> MTERTLKVLSPLHIGTGNELTPVDIYPRENIIHVLDTERLVNDLMNLGVELNEILALLKNPPGDAYIWKGYIEEFHLDPSDYSIYTLKIHGKIGRKSMQIKEFIKLNGRPYIPGSSLKGA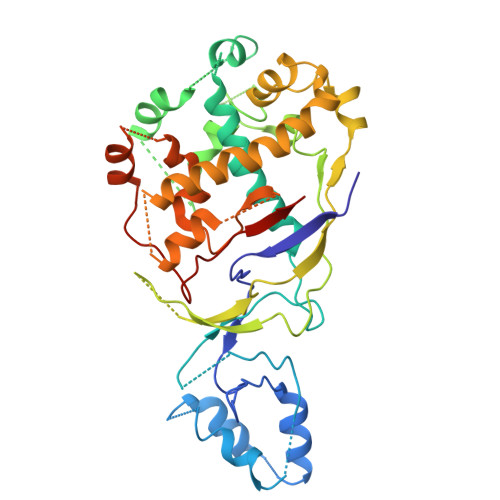IRTAVLYKALKECGDARAVMRVVSKVNGDVARDIGRSEDVLDYYMSFLSRARIDRKRADDLLEAIVFGMEPDRRSKIRYEPKRDPMKALIVRDSKPVGRKHLAVYHVEVIGNPQPIPIWVEAIEPGAATDVEIHVDTEALRLNADYFNGLLWECLKERGEPGEVFEDFLWEAVDEFYTAVMKYETIEVQKFGRYTSQVRSFYASLEDHSGHVLRLGWGSGWLAMTIGLLLVEKGYKWENVRKKLGLGKKPGGSGFSREFPKTRRLADGMPMGWVVLEHHHHHH>[2x]MAETPNSDMSGATGGRSKRPKSNQDWW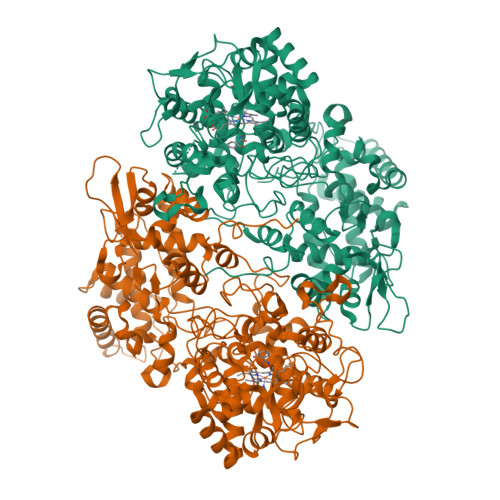PSKLNLEILDQNARDVGPVEDDFDYAEEFQKLDLEAVKSDLEELMTSSQDWWPADYGHYGPLFIRMAWHSAGTYRTADGRGGAAGGRQRFAPINSWPDNANLDKARRLLLPIKQKYGQKISWADLMILAGNVAIESMGFKTFGYAGGREDAFEEDKAVNWGPEDEFETQERFDEPGEIQEGLGASVMGLIYVNPEGPDGNPDPEASAKNIRQTFDRMAMNDKETAALIAGGHTFGKVHGADDPEENLGPEPEAAPIEQQGLGWQNKNGNSKGGEMITAGIEGPWTQSPTEWDMGYINNLLDYEWEPEKGPGGAWQWAPKSEELKNSVPDAHDPDEKQTPMMLTTDIALKRDPDYREVMETFQENPMEFGMNFAKAWYKLTHRDMGPPERFLGPEVPDEEMIWQDPLPDADYDLIGDEEIAELKEEILDSDLSVSQLVKTAWASASTYRDSDKRGGANGARLRLEPQKNWEVNEPEQLETVLGTLENIQTEFNDSRSDGTQVSLADLIVLGGNAAVEQAAANAGYDVEIPFEPGRVDAGPEHTDAPSFDALKPKVDGVRNYIQDDITRPAEEVLVDNADLLNLTASELTALIGGMRSIGANYQDTDLGVFTDEPETLTNDFFVNLLDMGTEWEPAADSEHRYKGLDRDTGEVKWEATRIDLIFGSNDRLRAISEVYGSADAEKKLVHDFVDTWSKVMKLDRFDLEHHHHHH>MRAMRLVEIGKPLKLEDIPIPKPKGSQVLIKIEAAGVCHSDVH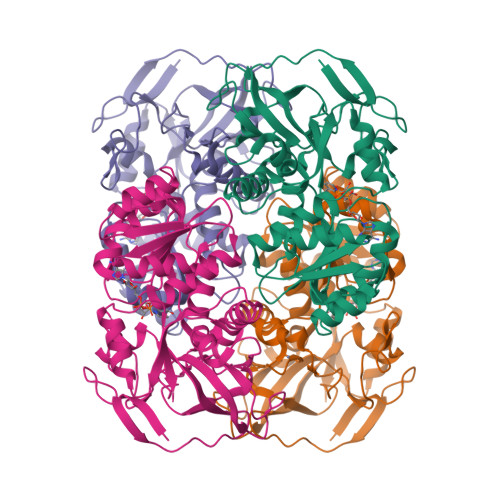MRQGRFGNLRIVEDLGVKLPVTLGHEIAGRIEEVGDEVVGYSKGDLVAVNPWEGEGNCYYCRIGEEHLCDSPRWLGINYDGAYAEYVLVPHYKYLYKLRRLSAVEAAPLTCSGVTTYRAVRKASLDPSKTLVVIGAGGGLGTMAIQIAKAVSGATIIGVDVREEALEAAKRAGADYVINASSQDPVSEIRRITQGKGADAVIDLNNSEKTLSIYPYVLAKQGKYVMVGLFGADLKYHAPLITLNEVQFIGSLVGNQSDFLGIMSLAEAGKVKPMVTKTMKLEEANEAIDNLENFKAVGRQVLVP[2x]>ARTDNFKLSSLANGLKVATSNTPGHFSALGLYIDAGSRFEGRNLKGCTHILDRLAFKSTEHVEGRAMAETLELLGGNYQCTSSRENLMYQASVFNQDVGKMLQLMSETVRFPKITEQELQEQKLSAEYEIDEVWMKPELVLPELLHTAAYSGETLGSPLICPRGLIPSISKYYLLDYRNKFYTPENTVAAFVGVPHEKALELTGKYLGDWQSTHPPITKKVAQYTGGESCIPPAPVFGNLPELFHIQIGFEGLPIDHPDIYALATLQTLLGGGGSFSAGGPGKGMYSRLYTHVLNQYYFVENCVAFNHSYSDSGIFGISLSCIPQAAPQAVEVIAQQMYNTFANKDLRLTEDEVSRAKNQLKSSLLMNLESKLVELEDMGRQVLMHGRKIPVNEMISKIEDLKPDDISRVAEMIFTGNVNNAGNGKGRATVVMQGDRGSFGDVENVLKAYGLGNSSSSKNDSPKKKGWFHHHHHH[4x];>ASQIPGTRTSKLPNGLTIATEYIPNTSSATVGIFVDAGSRAENVKNNGTAHFLQHLAFKGTQNRPQQGIELEIENIGSHLNAYTSRENTVYYAKSLQEDIPKAVDILSDILTKSVLDNSAIERERDVIIRESEEVDKMYDEVVFDHLHEITYKDQPLGRTILGPIKNIKSITRTDLKDYITKNYKGDRMVLAGAGAVDHEKLVQYAQKYFGHVPKSESPVPLGSPRGPLPVFCRGERFIKENTLPTTHIAIALEGVSWSAPDYFVALATQAIVGNWDRAIGTGTNSPSPLA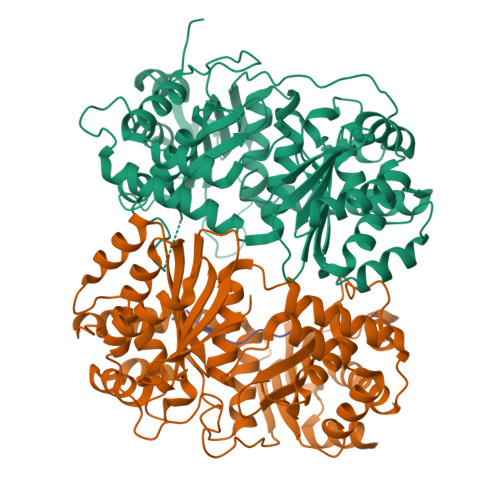VAASQNGSLANSYMSFSTSYADSGLWGMYIVTDSNEHNVRLIVNEILKEWKRIKSGKISDAEVNRAKAQLKAALLLSLDGSTAIVEDIGRQVVTTGKRLSPEEVFEQVDKITKDDIIMWANYRLQNKPVSMVALGNTSTVPNVSYIEEKLNQ[4x];>LSRVAKRA[4x]Here we describe the development of helical concave scaffolds tailored to the convex target sites typically involved in immune receptor interactions. We employed these scaffolds to design proteins that bind to TGFβRII, CTLA-4, and PD-L1, achieving low nanomolar to picomolar affinities and potent biological activity following experimental optimization. We focused on five-helix bundle scaffolds, with three helices forming the concave interface and two providing structural support. We reasoned that a set of concave helical scaffolds with shapes tailored to interact with a wide range of convex Ig fold-containing targets could provide starting points for the design of high-stability and affinity binders to immunotherapy targets.

We further optimized the most enriched design, 5HCS_TGFBR2_0, by resampling the sequences of interfacial residues in the bound state using ProteinMPNN25 and filtering the complex models using Alphafold220. Four of the most enriched optimized binders obtained after several rounds of yeast display selection were produced in E. coli. The highest affinity binder, 5HCS_TGFBR2_1, was found using biolayer interferometry to have an affinity less than 1 nM for TGFβRII (Fig. 2aand Supplementary Fig. 5a). We determined the co-crystal structures of 5HCS_TGFBR2_1 with TGFβRII. The high resolution (1.24 Å) X-ray crystal structure is very close to the computational design model (Fig. 2c; root mean square deviation (rmsd) over Cα atoms of 0.55 Å over the full complex), showing 5HCS_TGFBR2_1 binds to the TGF-β3 binding site on TGFβRII utilizing the concave surface as designed. Helices H1, H3, and H5 which form the concave binding surface interact with TGFβRII, and the most highly conserved non-core residues are in these helices. In H1, N10 hydrogen bonds with TGFβRII D142; in H3, S46 and S49 hydrogen bond to the backbone atoms of strand S72 - S75; and in H5, N93 hydrogen bonds to the backbone atoms of I76. A hydrophobic patch composed of F48, L50, and I76 on TGFβRII critical for TGF-β3 binding packs tightly on a hydrophobic groove formed by L6 from H1, M50, V52, K53 from H3 and V96, K99, V100 from H5. All the key interactions described above are recapitulated in the crystal structure with high side-chain orientation consistency. Design of such extended grooves and pockets is nearly impossible using small globular miniproteins; the high affinity binding and crystal structure of 5HCS_TGFBR2_1 demonstrates that 5HCS scaffolds can indeed be used to target convex binding sites. Dose-dependent inhibition of the TGFβ SMAD2/3 signaling was observed with an IC50 of 30.6 nM.

> SGSGLKELLKELNKAIASGDTETVRRILEELLELLKEAFEKGDYDLAISIASMAVKAASYIGDTETLKELLEILKKIKEKLKKEGDEAALKAVERNIKVVEKVA;> MKFPQLCKFCDVRFSTCDNQKSCMSNCSITSICEKPQEVCVAVWRKNDENITLETVCHDPKLPYHDFILEDAASPKCIMKEKKKPGETFFMCSCSSDECNDNIIFSEEYNT>[2x]HHHAIGYVWNTLYGWVDTGTGSLAAANLTARMQPISHHLAHPDTKRRFHELVCASGQIEHLTPIAAVAATDADILRAHSAAHLENMKRVSNLPTGGDTGDGITMMGNGGLEIARLSAGGAVELTRRVATGE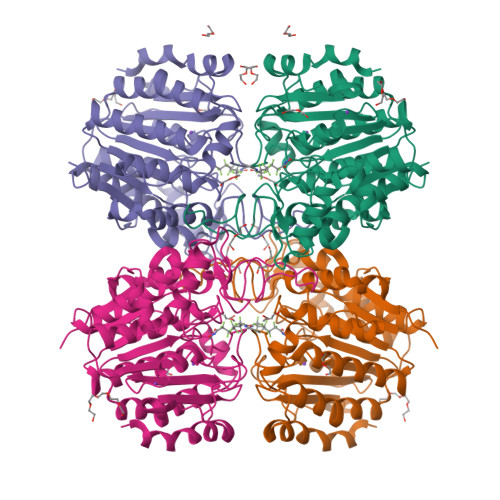LSAGYALVNPPGHHAPHNAAMGFCIFNNTSVAAGYARAVLGMERVAILDWDVHHGNGTQDIWWNDPSVLTISLHQHLCFPPDSGYSTERGAGNGHGYNINVPLPPGSGNAAYLHAMDQVVLPALRAYRPQLIIVGSGFDASMLDPLARMMVTADGFRQMARRTIDCAADICDGRIVFVQEGGYSPHYLPFCGLAVIEELTGVRSLPDPYHEFLAGMGGNTLLDAERAAIEEIVPLLADIR> MSALPEEVNRTLLQIVQAFASPDNQIRSVAEKALSEEWITENNIEYLLTFLAEQAAFSQDTTVAALSAVLFRKLALKAPITHIRKEVLAQIRSSLLKGFLSERADSIRHKLSDAIAECVQDDLPAWPELLQALIESLKSGNPNFRESSFRILTTVPYLITAVDINSILPIFQSGFTDASDNVKIAAVTAFVGYFKQLPKSEWSKLGILLPSLLNSLPRFLDDGKDDALASVFESLIELVELAPKLFKDMFDQIIQFTDMVIKNKDLEPPARTTALELLTVFSENAPQMCKSNQNYGQTLVMVTLIMMTEVSIDDDDAAEWIESDDTDDEEEVTYDHARQALDRVALKLGGEYLAAPLFQYLQQMITSTEWRERFAAMMALSSAAEGCADVLIGEIPKILDMVIPLINDPHPRVQYGCCNVLGQISTDFSPFIQRTAHDRILPALISKLTSECTSRVQTHAAAALVNFSEFASKDILEPYLDSLLTNLLVLLQSNKLYVQEQALTTIAFIAEAAKNKFIKYYDTLMPLLLNVLKVNNKDNSVLKGKCMECATLIGFAVGKEKFHEHSQELISILVALQNSDIDEDDALRSYLEQSWSRICRILGDDFVPLLPIVIPPLLITAKATQDVGLIEEEEAANFQQYPDWDVVQVQGKHIAIHTSVLDDKVSAMELLQSYATLLRGQFAVYVKEVMEEIALPSLDFYLHDGVRAAGATLIPILLSCLLAATGTQNEELVLLWHKASSKLIGGLMSEPMPEITQVYHNSLVNGIKVMGDNCLSEDQLAAFTKGVSANLTDTYERMQDRHGDGDEYNENIDEEEDFTDEDLLDEINKSIAAVLKTTNGHYLKNLENIWPMINTFLLDNEPILVIFALVVIGDLIQYGGEQTASMKNAFIPKVTECLISPDARIRQAASYIIGVCAQYAPSTYADVCIPTLDTLVQIVDFPGSKLEENRSSTENASAAIAKILYAYNSNIPNVDTYTANWFKTLPTITDKEAASFNYQFLSQ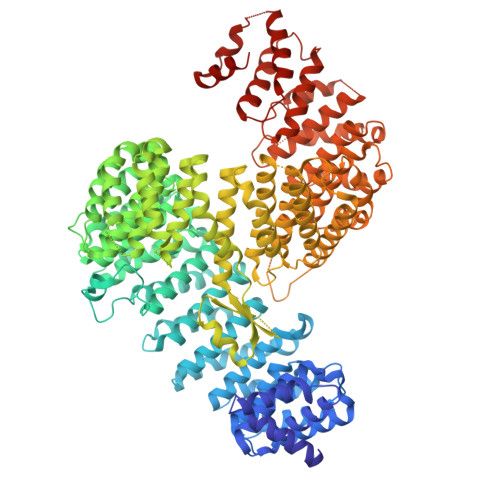LIENNSPIVCAQSNISAVVDSVIQALNERSLTEREGQTVISSVKKLLGFLPSSDAMAIFNRYPADIMEKVHKWFA> MPRPRVLLLGDPARHLDDLWSDFQQKFEVIPANLTTHDGFKQALREKRYGDFEAIIKLAVENGTESYPWNADLISHLPSSLKVFAAAGAGFDWLDLDALNERGVAFANSRGAGDTATSDLALYLILSVFRLASYSERAARTGDPETFNRVHLEIGKSAHNPRGHVLGAVGLGAIQKEIARKAVHGLGMKLVYYDVAPADA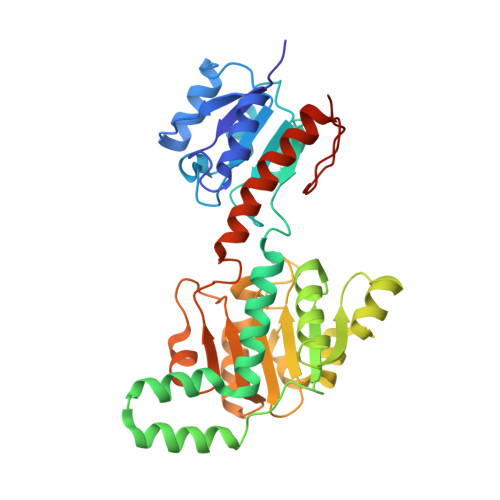ETEKALGAERVDSLEELARRSDCVSVSVPYMKLTHHLIDEAFFAAMKPGSRIVNTARGPVISQDALIAALKSGKLLSAGLDVHEFEPQVSKELIEMKHVTLTTHIGGVAIETFHEFERLTMTNIDRFLLQGKPLLTPAGKVFAPSSAA>[2x]GSHNMAEMVETVCGPVPVEQLGKTLIHEHFLFGYPG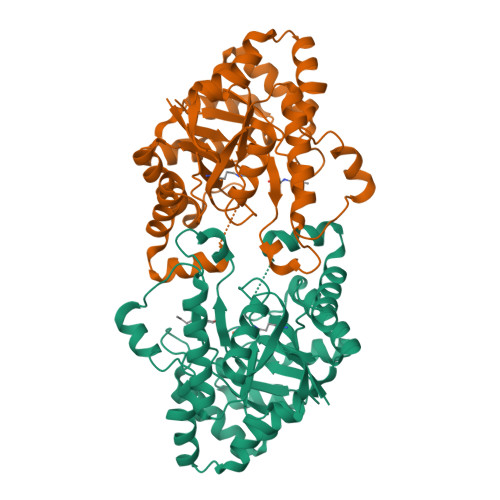FQGDVTRGTFREDESLRVAVEAAEKMKRHGIQTVVDPTPNDCGRNPAFLRRVAEETGLNIICATGYYYNGEGAPPYFQFRRLLGTAEDDIYDMFMAELTEGIADTGIKAGVIKLASSKGRITEYEKMFFRAAARAQKETGAVIITHTQEGTMGPEQAAYLLEHGADPKKIVIGHMCGNTDPDYHRKTLAYGVYIAFDRFGIQGMVGAPTDEERVRTLLALLRDGYEKQIMLSHNTVNVWLGRPFTLPEPFAEMMKNWHVEHLFVNIIPALKNEGIRDEVLEQMFIGNPAALFSA>[2x]GAMAQRMVWVDLEMTGLDIEKDQIIEMACLITDSDLNILAEGPNLIIKQPDELLDSMSDWCKEHHGK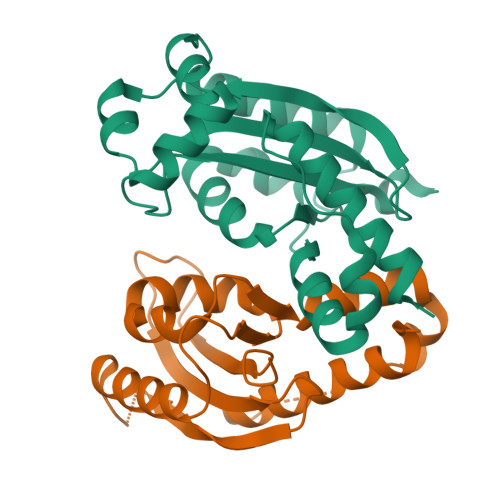SGLTKAVKESTITLQQAEYEFLSFVRQQTPPGLCPLAGNSVHEDKKFLDKYMPQFMKHLHYRIIDVSTVKELCRRWYPEEYEFAPKKAASHRALDDISESIKELQFYRNNIFK5,6,7,8-TETRAHYDRO-IMIDAZO[1,2-A]PYRIDINE-6,7,8-TRIOL | C7 H10 N2 O3 | 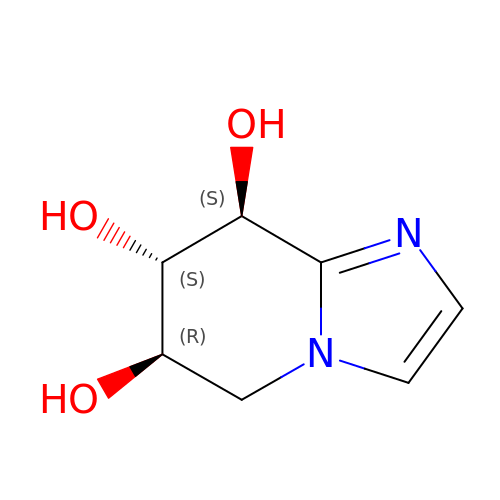QMHSBFMMOLGPGR-NGJCXOISSA-N>MGKSLSHLPLHSSKEDAYDGVTSENM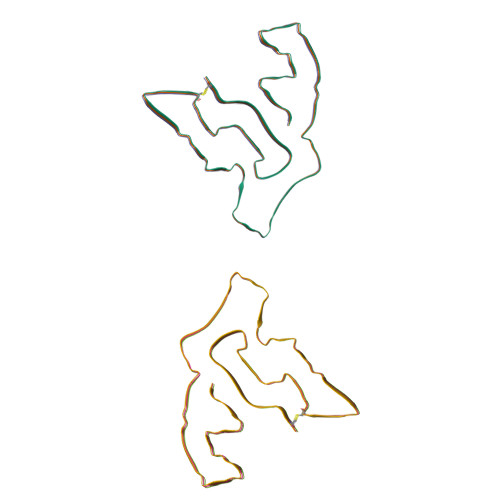RNGLVNSEVHNEDGRNGDVSQFPYVEFTGRDSVTCPTCQGTGRIPRGQENQLVALIPYSDQRLRPRRTKLYVMASVFVCLLLSGLAVFFLFPRSIDVKYIGVKSAYVSYDVQKRTIYLNITNTLNITNNNYYSVEVENITAQVQFSKTVIGKARLNNITIIGPLDMKQIDYTVPTVIAEEMSYMYDFCTLISIKVHNIVLMMQVTVTTTYFGHSEQISQERYQYVDCGRNTTYQLGQSEYLNVLQPQQ[6x]> MKVKINEVHSVFAWSWHIPSTSDEDAANNDPIGNDEDEDVCGICRASYNGTCPSCKFPGDQCPLVIGLCHHNFHDHCIYRWLDTPTSKGLCPMCRQTFQLQKGLAINDAHVQKFVEIVSRRREEMIEEGVAEEFVDFDEPIRQNTDNPIGRQQ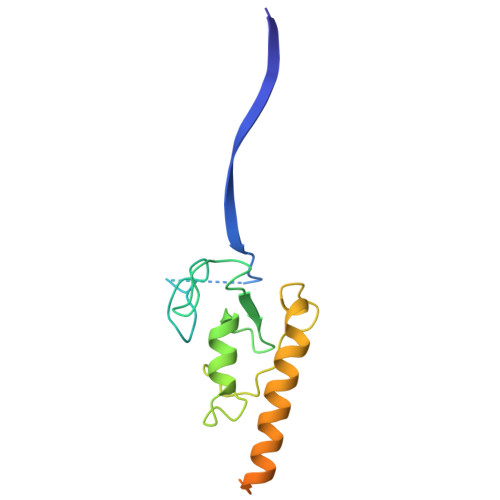VDTILDEDFLLR Y-family DNA polymerase κ (Pol κ) can replicate damaged DNA templates to rescue stalled replication forks. Access of Pol κ to DNA damage sites is facilitated by its interaction with the processivity clamp PCNA and is regulated by PCNA mono-ubiquitylation. In this work, we present cryo-EM reconstructions of full-length human Pol κ bound to a primer/template (P/T) DNA substrate, an incoming nucleotide, and wild-type PCNA (wt-PCNA) or PCNA mono-ubiquitylated at K164 (Ub-PCNA), at resolutions between ~3.4 and ~6.4 Å. The structures of the complexes with either wt-PCNA or Ub-PCNA are very similar and show the Pol κ core docked to one PCNA protomer through the internal PIP-box adjacent to the PAD.

Purified Ub-PCNA was mixed with Pol κ, the (25/38) P/T DNA containing a dideoxy chain terminator in the primer strand, and dTTP. Refinement of the main 3D class yielded a reconstruction of the Pol κ−DNA−Ub-PCNA complex at 3.7 Å resolution which is nearly identical to that obtained with unmodified PCNA (RMSDCα ~ 0.5 Å), and where the ubiquitin moieties are not visible. A different 3D class showed residual density protruding radially away from the back face of PCNA where the three lysine residues at position 164 are located. Refinement of this class yielded a map at 6.4 Å resolution, which was further improved by density modification implemented in Phenix44 (Fig. 4a−c and Supplementary Fig. 7). Additional differences compared to the reconstruction of the complex with wt-PCNA are the appearance of a rod-shaped density corresponding to αN1 of the N-clasp of Pol κ, and a slight tilt (~5°) of the catalytic domain towards the PCNA monomer bound to Pol κ. Density at the ubiquitin positions is weak and the map local resolution lower than the average, implying that the ubiquitins covalently attached to PCNA retain a significant degree of flexibility. However, the density protruding from the PCNA monomer bound to Pol κ is better defined and displays the characteristic barrel-shape of ubiquitin (Ub1, Fig. 4a−c). However, due to the weak map density and local resolution in the Ub1 region, we cannot exclude that ubiquitin may exist in multiple orientations which the cryo-EM reconstruction could not resolve. The outward location of ubiquitin density implies the exposure of the ubiquitin hydrophobic patch to interact with Pol κ UBZs, but the map features are at odds with the existence of a rigid Ub/UBZ complex (Fig. 4a−c), suggesting that the Ub/UBZ interaction is transient and/or involves multiple ubiquitin and UBZ conformations. Our cryo-EM structure of PCNA enzymatically mono-ubiquitylated at K164 in complex with both Pol κ and DNA shows that the orientation of Pol κ relative to PCNA is dictated by the PIP-box and DNA interactions, and that the three ubiquitins are partly flexible and extend away from the PCNA ring.

> MDSTKEKCDSYKDDLLLRMGLNDNKAGMEGLDKEKINKIIMEATKGSRFYGNELKKEKQVNQRIENMMQQKAQITSQQLRKAQLQVDRFAMELEQSRNLSNTIVHIDMDAFYAAVEMRDNPELKDKPIAVGSMSMLSTSNYHARRFGVRAAMPGFIAKRLCPQLIIVPPNFDKYRAVSKEVKEILADYDPNFMAMSLDEAYLNITKHLEERQNWPEDKRRYFIKMGSSVENDNPGKEVNKLSEHERSISPLLFEESPSDVQPPGDPFQVNFEEQNNPQILQNSVVFGTSAQEVVKEIRFRIEQKTTLTASAGIAPNTMLAKVCSDKNKPNGQYQILPNRQAVMDFIKDLPIRKVSGIGKVTEKMLKALGIITCTELYQQRALLSLLFSETSWHYFLHISLGLGSTHLTRDGERKSMSVERTFSEINKAEEQYSLCQELCSELAQDLQKERLKGRTVTIKLKNVNFEVKTRASTVSSVVSTAEEIFAIAKELLKTEIDADFPHPLRLRLMGVRISSFPNEEDRKHQQRSIIGFLQAGNQALSATECTLEKTDKDKFVKPLEMSHKKSFFDKKRSERKWSHQDTFKCEAVNKQSFQTSQPFQVLKKKMNENLEISENSDDCQILTCPVCFRAQGCISLEALNKHVDECLDGPSISENFKMFSCSHVSATKVNKKENVPASSLCEKQDYEAHPKIKEISSVDCIALVDTIDNSSKAESIDALSNKHSKEECSSLPSKSFNIEHCHQNSSSTVSLENEDVGSFRQEYRQPYLCEVKTGQALVCPVCNVEQKTSDLTLFNVHVDVCLNKSFIQELRKDKFNPVNQPKESSRSTGSSSGVQKAVTRTKRPGLMTKYSTSKKIKPNNPKHTLDIFFK;>[3x]GPHMFEARLVQGSILKKVLEALKDLINEACWDISSSGVNLQSMDSSHVSLVQLTLRSEGFDTYRCDRNLAMGVNLTSMSKILKCAGNEDIITLRAEDNADTLALVFEAPNQEKVSDYEMKLMDLDVEQLGIPEQEYSCVVKMPSGEFARICRDLSHIGDAVVISCAKDGVKFSASGELGNGNIKLSQTSNVDKEEEAVTIEMNEPVQLTFALRYLNFFTKATPLSSTVTLSMSADVPLVVEYKIADMGHLKYYLAPKIEDEEGS>[2x]MIIGTYRLQLNKGFTFYDTIENLDYFKELGVSHLYLSPILKARPGSTHGYDVVDHSEINEELGGEEGYFKLVKEAKSRGLEIIQDIVPNHMAVHHTNWRLMDLLKSWKNSKYYNYFDHYDDDKIILPILEDELDTVIDKGLIKLQKDNIEYRGLVLPINDEGVEFLKRINCFDNSCLKKEDIKKLLLMQYYQLTYWKKGYPNYRRFFAVNDLIAVRIELDEVFRESHEIIAKLPVDGLRIDHIDGLYNPKEYLDKLRQLVGNDKIIYVEKILSINEKLRDDWKVDGTTGYDFLNYVNMLLVDGSGEEELTKFYENFIGRKINIDELIIQSKKLVANQLFKGDIERLSKLLNVNYDYLVDFLACMKKYRTYLPFEDINGIRECDKEGKLKDEKGIMRLQQYMPAIFAKGYEDTTLFIYNRLISLNEV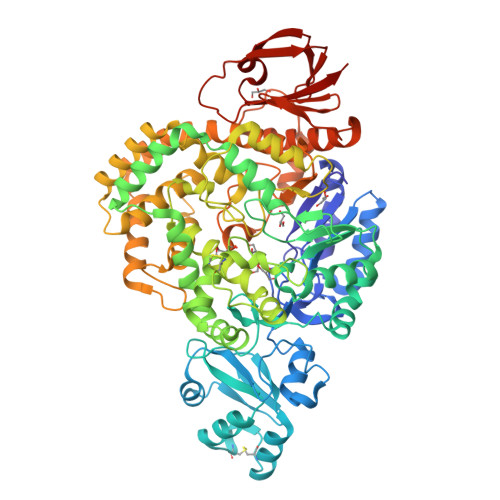GSDLRRFSLSIEDFHNFNLSRVNTISMNTLSTHDTKFSEDVRARISVLSEIPKEWEERVKYWHDLLRPNIDKNDEYRFYQTLVGSYEGFDNKERIKNHIIKVIREAKVHTTWENPNLEYEKKVLGFIDEVFENSSFRNDFDNFEKKIVYFGYMKSLVATTLKFLSPGVPDIYQGTEVWRFLLTDPDNRMAVDFRKLRELLNNLTEKNLELSDPRTKMLYVKKLLQLRREYSLNDYKPLPFGFQRGKVTVLFSPIVTREVKEKISIRQKSVDWIRNEEISSGEYNLSELIGEHKVVILTEKRE~{N}-[5-[6-[(dimethylamino)methyl]-2,3-dihydro-1,4-benzoxazin-4-yl]-2-methoxy-pyridin-3-yl]methanesulfonamide | C18 H24 N4 O4 S | 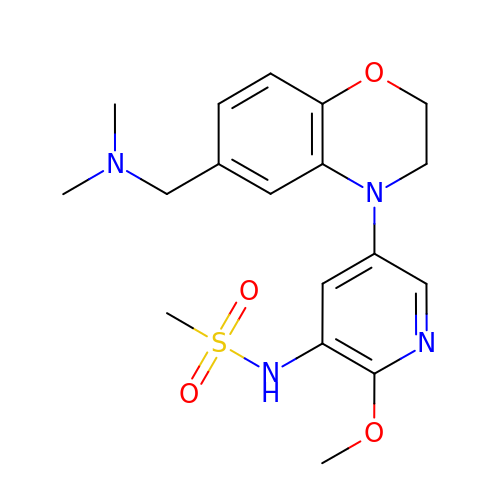SAHCNYAOSGATSF-UHFFFAOYSA-N>MSRPVSDTMAALMAKGKTAFIPYITAGDPDLATTAEALRLLDGCGADVIELGVPCSDPYIDGPIIQASVARAL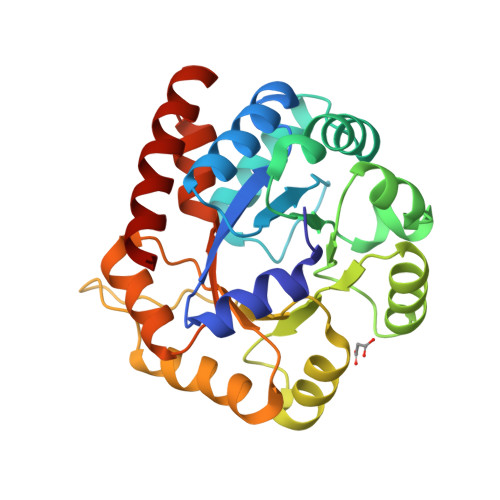ASGTTMDAVLEMLREVTPELSCPVVLLSYYKPIMFRSLAKMKEAGVHGLIVPDLPYVAAHSLWSEAKNNNLELVLLTTPAIPEDRMKEITKASEGFVYLVSVNGVTGPRANVNPRVESLIQEVKKVTNKPVAVGFGISKPEHVKQIAQWGADGVIIGSAMVRQLGEAASPKQGLRRLEEYARGMKNALG[2x]5-BETA-D-RIBOFURANOSYLPICOLINAMIDE 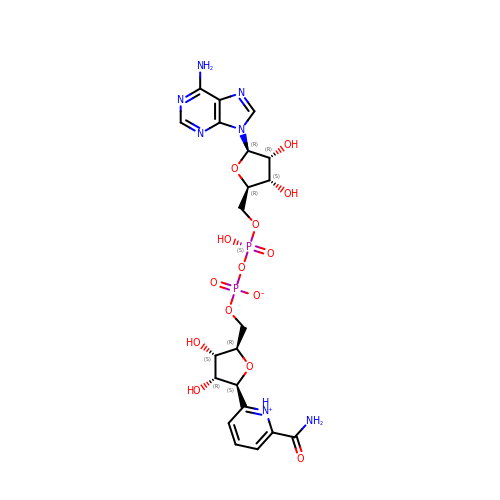ADENINE-DINUCLEOTIDE | C21 H27 N7 O14 P2 | LFERELMXERXKKQ-KMXXXSRASA-N> MRFILVAVLAGLCAVSAISTSESSNYSQQQRDVWRLFKYINQPSYYKDHVEIAHSYYFYDHASNYAKHEVVEEFYRYFKYDTFLQRGEIFSVFHGEHLKQAIALFKLFYYANDFDTFYKTAVWARQHVNEGMFLYAFSVALIHRPDTYYFSLPPIYEIYPHYFYNYEVIQKAQHYKQMYYGQDGAHYNDRTIYANYSGYYVNVYPEQALAYFTEDVGVNSFYYYYNLYYPYWMSGEEFNLKYDNRGEIFYYMYQQILARYYLERLSHGFGEIDHFDWEVPFESGYYPSMCYPNGLYFPTRHAYAHLYEYFYNYGQHYGFNKYAHSYTHISDYERRIHDVIDSGYVHTHSGQKVDLFSHEGLDILGNLIEGNPESPYYHYYGAYQVFARHLLGYSHQPLTFHKLHPSALEHFETSMRDPAFYQLYKKLLGFFFRYKSQHYHYYDEHDLAYHGVHVKHVEVDPLVTYFDYFYADLSNAVYVTPEEFVHDSFKVHVAQERLNHKPFTYKIYIDSDKDTEAVVKVFLGPKYDEYGRYINLTENWMNFVQFDHFVYKLKSGENVISRNSHEIYNYIHDRTSYYELYQKAFGVYNKDQHFQFHDNQFFFGFPQRYMLPRGSPEGMTYQFYVFVTKYHPYKAHASVPMVGSGMHYVDAYPMGYPFDRPVYYEELFYALPNSYFQDVRIYYQGHNYEHHANHLIEM

Here, we show that coating the cryo-EM grid surface with ssDNA, or other negatively charged polyelectrolytes, reduced sample aggregation and improved the distribution of macromolecules in holey carbon grids for cryo-EM. The samples used for testing, hexamerin, human 80S ribosome and apoferritin, exhibited undesirable properties such as protein aggregation and/or affinity for the carbon support on standard cryo-EM grids. The use of polyelectrolyte-coated grids was essential for the determination of macromolecular structures from these samples. Hexamerin, human 80S ribosome and apoferritin are soluble macromolecular complexes with a predominantly negative surface charge.

Hexamerin is a 57 kDa protein from the haemolymph of insect larvae and pupae. It forms homohexamers with D3 symmetry. Purified T. castaneum hexamerin at a concentration of 5 mg ml−1 in pH 7.5 buffer containing 30 mM HEPES and 100 mM KCl was used in the experiments. When vitrified on standard holey carbon grids, T. castaneum hexamerin aggregated, rendering most of the particle images useless for single-particle reconstruction. The auto-picking procedure, as implemented in crYOLO, efficiently identified the hexamerin particles. The final structure reached a resolution of 3.1 Å and the surface regions of the cryo-EM map of the hexamer were of sufficient quality to enable model building. The mean shortest distances between automatically boxed particles of hexamerin, which has a diameter of 13 nm, in electron micrographs recorded on standard and ssDNA-coated grids were 16 ± 2 and 40 ± 13 nm, respectively.>MGQNMEIDNFLKIERLAENDLPKFIQLIRLFEAVFEMKNFSIPDSEHLQKLLNQNNFYVFVALLENKIVGGLTSYVLEQYYSEKPLAYIYDLAVDTNWQRQGIGKKLITATNQFYTEKGFEEVFVQADKVDDYALDFYRSTK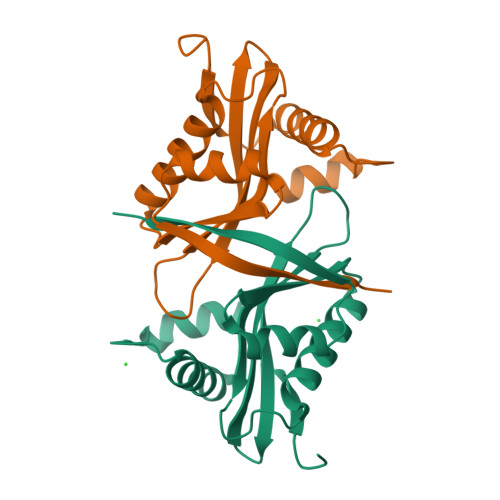PTAEEQVVHFYYTLK[2x]> GPEFMAFSELLDLVGGLGRFQVLQTMALMVSIMWLCTQSMLENFSAAVPSHRCWAPLLDNSTAQASILGSLSPEALLAISIPPGPNQRPHQCRRFRQPQWQLLDPNATATSWSEADTEPCVDGWVYDRSIFTSTIVAKWNLVCDSHALKPMAQSIYLAGILVGAAVCGPASDRFGRRLVLTWSYLQMAVSGTAAAFAPTFPVYCLFRFLLAFAVAGVMMNTGTLLMEWTSARARPLVMTLNSLGFSFGHGLTAAVAYGVRDWTLLQLAVSVPFFLCFLYSWWLAESARWLLTTGRLDRGLQELRRVAAINGKRAVQDTLTPEVLLSAMREELSVGQAPASLGTLLRTPGLRLRTCISTLCWFAFGFTFFGLALDLQALGSNIFLLQVLIGVVDIPAKMGALLLLSRLGRRPTLAASLLLAGLCILANTLVPHEMGALRSALAVLGLGGVGAAFTCITIYSSELFPTVLRMTAVGLGQMAARGGAILGPLVRLLGVHGPWLPLLVYGTVPVLSGLAALLLP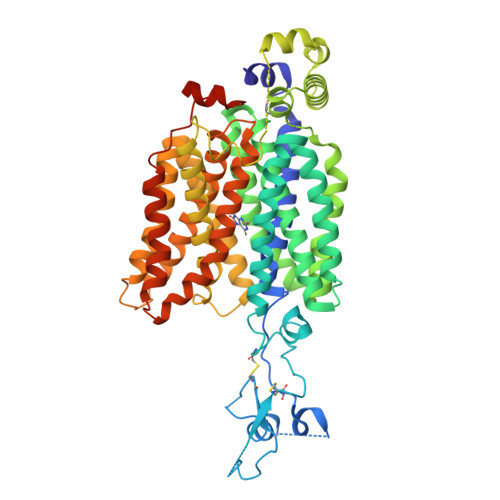ETQSLPLPDTIQDVQNQAVKKATHGTLGNSVLKSTQF>[3x]MHHHHHHSSGLVPRGSMILHAQAKHGKPGLPWLVFLHGFSGDCHEWQEVGEAFADYSRLYVDLPGHGGSAAISVDGFDDVTDLLRKTLVSYNILDFWLVGYSLGGRVAMMAACQGLAGLCGVIVEGGHPGLQNAEQRAEAQRSDRQWVQRFLTEPLTAVFADWYQQPVFASLNDDQRRELVALRSNNNGATLAAMLEATSLAVQPDLRANLSARTFAFYYLCGERDSKFRALAAELAADCHVIPRAGHNAHRENPAGVIASLAQILRF

Re-annotation of the activity of an earlier enzyme in the pathway, MenD, then led to the recognition that the true enzymatic activity of MenH is to covert the MenD reaction product, 2-succinyl-5-enolpyruvyl-6-hydroxy-3-cyclohexene-1-carboxylate (SEPHCHC) to 2-succinyl-6-hydroxy-2,4-cyclohexadiene-1-carboxylate (SHCHC) by a 2,5 elimination of pyruvate from the cyclohexene ring. MenH is thus correctly annotated as SHCHC synthase. EcMenH adopts a typical α/β-hydrolase fold, comprising a core β-sheet of mostly parallel strands surrounded on both sides by α-helices. As is characteristic of the α/β-hydrolases the three catalytic triad residues (Ser86, His232, Asp210) are located on loops of the core α/β–domain.

Accordingly, we report the structure of the MenH from E. coli at 2.75 Å resolution, along with the structures of two active site mutant enzymes, Arg124Ala and Tyr85Phe, both at 2.5 Å resolution. Structural comparisons of native EcMenH with the two mutant structures, R124A and Y85F using SSM shows they overlay very closely, with rms differences of 0.26–0.61 Å in Cα-atom positions over the entire structure. This shows that the mutations do not affect the polypeptide conformation significantly. The active sites differ very little, apart from weaker density for the sulfate ion in the R124A structure, due to the loss of the Arg124 interactions. Arg124 is held in place by a hydrogen bond between NE and the carboxyl group of Asp128, but has its NH1 and NH2 groups pointing out into the middle of the cavity. The sulfate ion forms hydrogen bonded ion pairs with both Arg90 and Arg124, which appear to be the primary determinants of binding. The main difference for the R124A mutant is that much more variability is seen in the orientation of the pyruvate group, with the loss of the guanidinium group of Arg124. Two conserved basic residues, Arg90 and Arg124, are in position to bind the carboxyl groups of the enol-pyruvyl group and the cyclohexenyl ring, with Arg90 having a particularly important role. Arg124 projects out into the active site from the lid domain, held in position by a hydrogen bond with Asp128. The structure is not perturbed by the mutations.>[2x]MNYPAEPFRIKSVETVSMIPRDERLKKMQEAGYNTFLLNSKDIYIDLLTDSGTNAMSDKQWAGMMMGDEAYAGSENFYHLERTVQELFGFKHIVPTHQGRGAENLLSQLAIKPGQYVAGNMYFTTTRYHQEKNGAVFVDIVRDEAHDAGLNIAFKGDIDLKKLQKLIDEKGAENIAYICLAVTVNLAGGQPVSMANMRAVRELTAAHGIK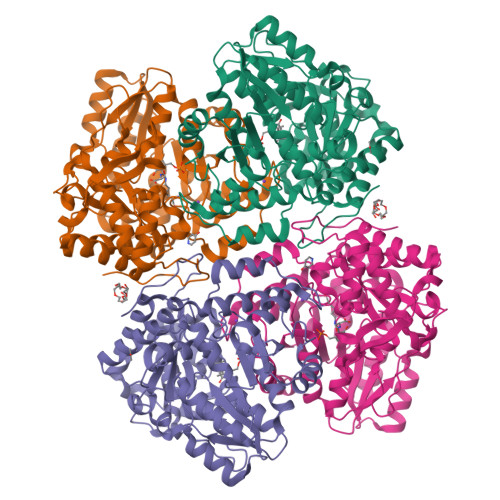VFYDATRCVENAYFIKEQEQGFENKSIAEIVHEMFSYADGCTMSGKKDCLVNIGGFLCMNDDEMFSSAKELVVVYEGMPSYGGLAGRDMEAMAIGLREAMQYEYIEHRVKQVRYLGDKLKAAGVPIVEPVGGHAVFLDARRFCEHLTQDEFPAQSLAASIYVETGVRSMERGIISAGRNNVTGEHHRPKLETVRLTIPRRVYTYAHMDVVADGIIKLYQHKEDIRGLKFIYEPKQLRFFTARFDYI> MEFFGESWKKHLSGEFGKPYFIKLMGFVAEERKHYTVYPPPHQVFTWTQMCDIKDVKVVILGQDPYHGPNQAHGLCFSVQRPVPPPPSLENIYKELSTDIEDFVHPGHGDL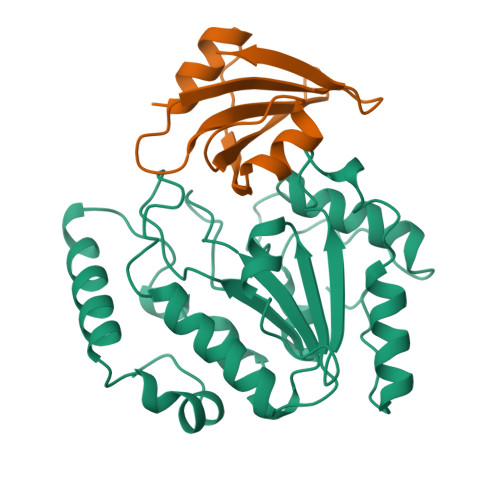SGWAKQGVLLLNAVLTVRAHQANSHKERGWEQFTDAVVSWLNQNSNGLVFLLWGSYAQKKGSAIDRKRHHVLQTAHPSPLSVYRGFFGCRHFSKTNELLQKSGKKPIDWKEL;> NLSDIIEKETGKQLVIQESILMLPEEVEEVIGNKPESDILVHTAYDESTDENVMLLTSDAPEYKPWALVIQDSNGENKIKML>MSMSQFFIRRPVFAWVIAIFIIIFGLLSIPKLPIARFPSVAPPQVNISATYPGATAKTINDSVVTLIERELSGVKNLLYYSATTDTSGTAEITATFKPGTDVEMAQVDVQNKIKAVEARLPQVVRQQGLQVEASSSGFLMLVGINSPNNQYSEVDLSDYLVRNVVEELKRVEGVGKVQSFGAEKAMRIWVDPNKLVSYGLSISDVNNAIRENNVEIAPGRLGDLPAEKGQLITIPLSAQGQLSSLEQFKNISLKSKTNGSVIKLSDVANVEIGSQAYNFAILENGKPATAAAIQLSPGANAVKTAEGVRAKIEELKLNLPEGMEFSIPYDTAPFVKISIEKVIHTLLEAMVLVFIVMYLFLHNVRYTLIPAIVAPIALLGTFTVMLLAGFSINVLTMFGMVLAIGIIVDDAIVVVENVERIMATEGLSPKDATSKAMKEITSPIIGITLVLAAVFLPMAFASGSVGVIYKQFTLTMSVSILFSALLALILTPALCATILKPIDGHHQKKGFFAWFDRSFDKVTKKYELMLLKIIKHTVPMMVIFLVITGITFAGMKYWPTAFMPEEDQGWFMTSFQLPSDATAERTRNVVNQFENNLKDNPDVKSNTAILGWGFSGAGQNVAVAFTTLKDFKERTSSASKMTSDVNSSMANSTEGETMAVLPPAIDELGTFSGFSLRLQDRANLGMPALLAAQDELMAMAAKNKKFYMVWNEGLPQGDNISLKIDREKLSALGVKFSDVSDIISTSMGSMYINDFPNQGRMQQVIVQVEAKSRMQLKDILNLKVMGSSGQLVSLSEVVTPQWNKAPQQYNRYNGRPSLSIAGIPNFDTSSGEAMREMEQLIAKLPKGIGYEWTGISLQEKQSESQMAFLLGLSMLVVFLVLAALYESWAIPLSVMLVVPLGIFGAIIAIMSRGLMNDVFFKIGLITIIGLSAKNAILIVEFAKMLKEEGMSLIEATVAAAKLRLRPILMTSLAFTCGVIPLVIATGASSETQHALGTGVFGGMISATILAIFFVPVFFIFILGAVEKLFSSKKKISSALEVLFQGPHHHHHHHHHH[3x]

Upon antibiotic stress Gram-negative pathogens deploy resistance-nodulation-cell division-type tripartite efflux pumps. These include a H+/drug antiporter module that recognizes structurally diverse substances, including antibiotics. The superfamily of resistance-nodulation-cell division (RND) efflux pumps plays a key role in intrinsic MDR in Gram-negative bacteria. These tripartite complexes comprise an RND transporter in the inner membrane that acts as a secondary active H+/drug antiporter extruding a vast spectrum of structurally unrelated drugs through a periplasmic membrane fusion protein channel connected to an outer membrane channel factor across the outer membrane. A comparison between drug binding of AdeB and Escherichia coli AcrB is made via activity analysis of 20 AdeB variants, selected on basis of side chain interactions with antibiotics observed in the AcrB periplasmic domain X-ray co-structures with fusidic acid (2.3 Å), doxycycline (2.1 Å) and levofloxacin (2.7 Å).

For structural elucidation of this RND transporter, we reconstituted AdeB in Salipro Nanodiscs sustaining a native-like lipid environment. Here, we show the single-particle cryo-EM structure of trimeric AdeB in the OOO conformation and in the L*OO conformation. A C3-symmetric density map could be solved up to a resolution of 3.5 Å. The AdeB trimer adopts mainly a resting state with all protomers in a conformation devoid of transport channels or antibiotic binding sites. All entry sites are closed in the O conformation, and an exit channel is opened. In the O conformation, the PC1 and PC2 subdomains are in close contact constituting a closed cleft. As observed in structures of AcrB, the closure of these entry tunnels appears concomitant with the opening of an exit tunnel in the O conformation of AdeB. Our single-particle cryo-EM results in this work show that 90% of imaged AdeB protomers remain inaccessible to substrates from the periplasm in the O conformation. We assume that the high prevalence of particles in the OOO conformation is not an artifact, as similar trimeric conformations have been observed in another cryo-EM structure of AdeB29 and a crystal structure of Campylobacter jejuni CmeB43. Whereas it is not possible to discern whether the L* conformation is recurring in the postulated AdeB LTO cycle, that state appears to be the only one bearing entrances from the periplasm in the absence of substrates. This would allow initial substrate entry in case drugs enter the periplasm, since the OOO state lacks substrate entry and binding sites.>[2x]MSKPQPIAAANWKCNGSQQSLSELIDLFNSTSINHDVQCVVASTFVHLAMTKERLSHPKFVI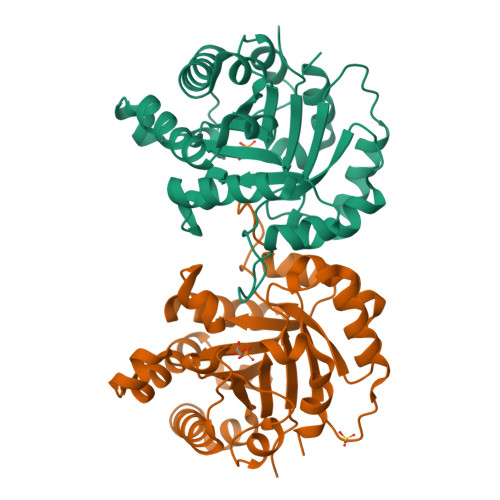AAQNAIAKSGAFTGEVSLPILKDFGVNWIVLGHSERRAYYGETNEIVADKVAAAVASGFMVIACIGETLQERESGRTAVVVLTQIAAIAKKLKKADWAKVVIAYEAVWAIGTGKVATPQQAQEAHALIRSWVSSKIGADVAGELRILYGGSVNGKNARTLYQQRDVNGFLVGGASLKPEFVDIIKATQ> MSGEEERKEKREKVRAGLKRAIAELPAEVAARCLALLDDASDEEFIEAVLEVLEAMREALVAMAREGRLDAVRRATSHINEVLVDAAELALEKGREYFRRLCLIVCDMMIELIRLEPEQTPELRRIRERLEEIRRRLEGSG;> DMRPEIWIAQELRRIGDEFNAYYAR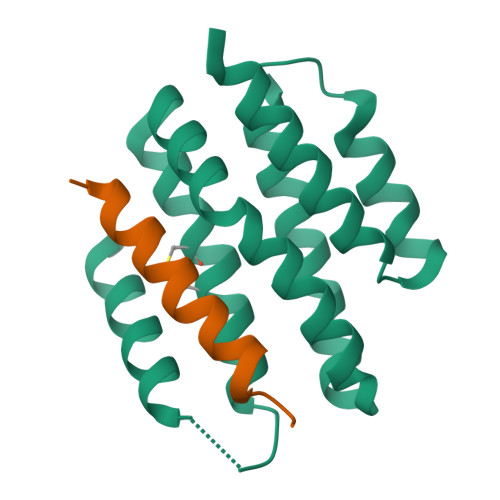R> NVPEIKAKEVNVDD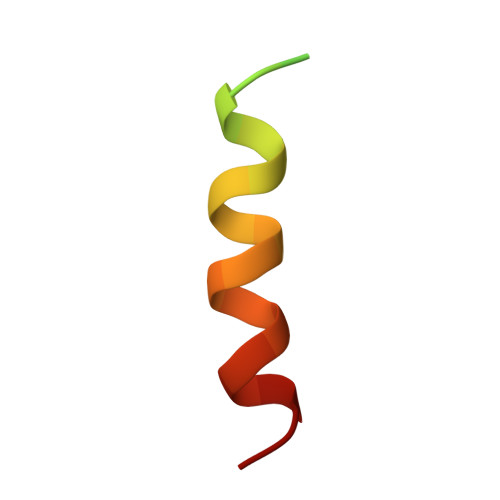EKEDKLAQRLRALRG> LPAHLQQTFSPEEIQFIVENEPIKIFPRITTRQKIRGDDRGTGNHTRWQLITTDDKALNNMVAMRSTEVVLWIALLLKQQSKCSIVAPQWLTTKELDRKIQYEKTHPDRFSELPW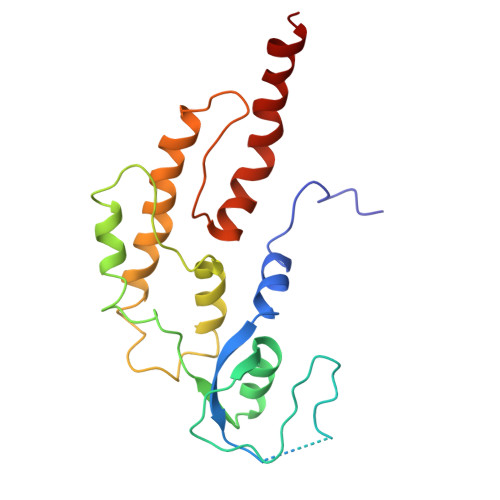NWLVLARILFNKAKDDFHDPIHELRGKIQDLREIRQIKVLKGLKYLNESHLQLDNLSLLEINELRPFITEIMDKLREIHTASL>MEDDPVWRFDDRDVILYNIALGATTKQLKYVYENDSDFQVIPTFGHLITFNSGKSQNSFAKLLRNFNPMLLLHGEHYLKVHSWPPPTEGEIKTTFEPIATTPKGTNVVIVHGSKSVDNKSGELIYSNEATYFIRNCQADNKVYADRPAFATNQFLAPKRAPDYQVDVPVSEDLAALYRLSGDRNPLHIDPNFAKGAKFPKPILHGMCTYGLSAKALIDKFGMFNEIKARFTGIVFPGETLRVLAWKESDDTI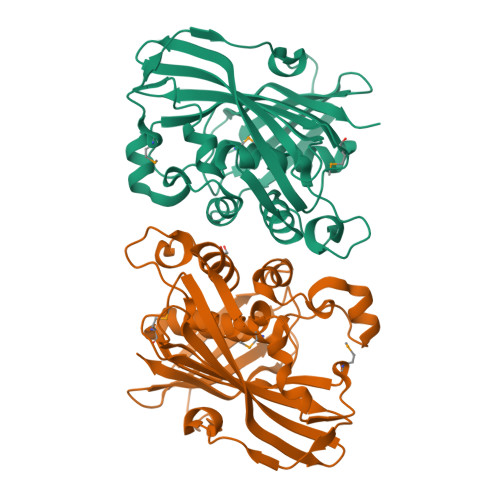VFQTHVVDRGTIAINNAAIKLVGDKAKI[4x]> MPANDFVSPDSIRAQFSAAMSLMYKQEVPLYGTLLELVSEINQQVMAQQPEVAEALRWTGEIERLDQERHGAIRVGTAEELATIARLFAVMGMQPVGYYDLSSAGVPVHSTAFRAVHEQSLHVSPFRVFTSLLRLELIDNPQLRELAQSILAKRQIFTSRALELIAQCEREGGLDAADAETFVQEALHTFRWHQDATVTAEQYQQLHDQHRLIADVVAFKGPHINHLTPRTLDIDAIQLGMPAKGIPPKAVVEGPPTRRHPILLRQT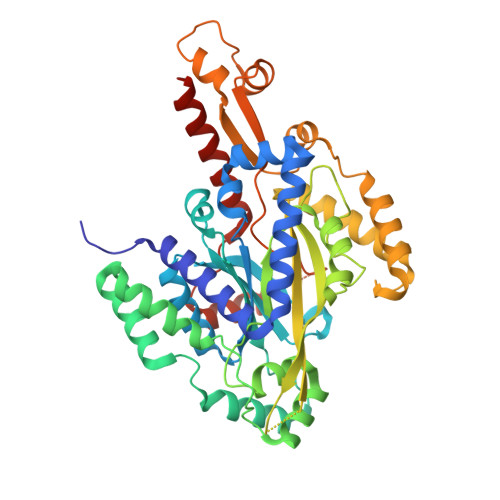SFKALQETVAFRDQQGREGSHTARFGEIEQRGAALTPKGRQLYDKLLDATRVALGGAPAEANAERYMALLQANFAEFPDDLAQMREQGLAYFRYFATEKGLAARDQEGRPTTLQGLIDAGHVHFEALVYEDFLPVSAAGIFQSNLGDDAQAEYGSNANREAFEAALGLQVQDELALYAQSERRSLQACAQALNLGSM> APVRSLNATLRDSQQKSLVMSGPYELKALHLQGQDMEQQVVFSMSFVQGEESNDKIPVALGLKEKNLYLSCVLKDDKPTLQLESVDPKNYPKKKMEKRFVFNKIEINNKLEFESAQFPNWYISTSQ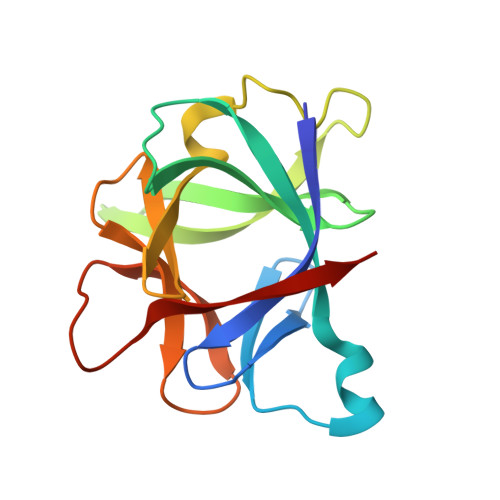AENMPVFLGGTKGGQDITDFTMQFVSS>MKRNYILGLDIGITSVGYGIIDYETRDVIDAGVRLFKEANVENNEGRRSKRGARRLKRRRRHRIQRVKKLLFDYNLLTDHSELSGINPYEARVKGLSQKLSEEEFSAALLHLAKRRGVHNVNEVEEDTGNELSTKEQISRNSKALEEKYVAELQLERLKKDGEVRGSINRFKTSDYVKEAKQLLKVQKAYHQLDQSFIDTYIDLLETRRTYYEGPGEGSPFGWKDIKEWYEMLMGHCTYFPEELRSVKYAYNADLYNALNDLNNLVITRDENEKLEYYEKFQIIENVFKQKKKPTLKQIAKEILVNEEDIKGYRVTSTGKPEFTNLKVYHDIKDITARKEIIENAELLDQIAKILTIYQSSEDIQEELTNLNSELTQEEIEQISNLKGYTGTHNLSLKAINLILDELWHTNDNQIAIFNRLKLVPKKVDLSQQKEIPTTLVDDFILSPVVKRSFIQSIKVINAIIKKYGLPNDIIIELAREKNSKDAQKMINEMQKRNRQTNERIEEIIRTTGKENAKYLIEKIKLHDMQEGKCLYSLEAIPLEDLLNNPFNYEVDHIIPRSVSFDNSFNNKVLVKQEENSKKGNRTPFQYLSSSDSKISYETFKKHILNLAKGKGRISKTKKEYLLEERDINRFSVQKDFINRNLVDTRYATRGLMNLLRSYFRVNNLDVKVKSINGGFTSFLRRKWKFKKERNKGYKHHAEDALIIANADFIFKEWKKLDKAKKVMENQMFEEKQAESMPEIETEQEYKEIFITPHQIKHIKDFKDYKYSHRVDKKPNRELINDTLYSTRKDDKGNTLIVNNLNGLYDKDNDKLKKLINKSPEKLLMYHHDPQTYQKLKLIMEQYGDEKNPLYKYYEETGNYLTKYSKKDNGPVIKKIKYYGNKLNAHLDITDDYPNSRNKVVKLSLKPYRFDVYLDNGVYKFVTVKNLDVIKKENYYEVNSKCYEEAKKLKKISNQAEFIASFYNNDLIKINGELYRVIGVNNDLLNRIEVNMIDITYREYLENMNDKRPPRIIKTIASKTQSIKKYSTDILGNLYEVKSKKHPQIIKKG[2x];>SMRKTIERLLNSELSSNSIAVRTGVSQAVISKLRNGKKELGNLTLNSAEKLFEYQKEMEKVDTWIVYRGRTADMNKSYIAEGSTYEEVYNNFVDKYGYDVLDEDIYEIQLLKKNGENLDDYDVDSDGINNYDKLDEFRESDYVDLEDYDYRELFENSSSQVYYHEFEITHE[2x]

AcrIIA15 is an anti-CRISPR (Acr) protein that inhibits Staphylococcus aureus Cas9 (SaCas9). The AcrIIA15 protein, consisting of 170 amino acids, is comprised of two domains: an N-terminal domain (NTD) from residues 1 to 56, which contains a HTH motif resembling a transcriptional repressor, and a C-terminal domain (CTD) from residues 57 to 170. AcrIIA15, by combining the HTH domain and Cas9 inhibitory domain within a single protein, exhibits dual functionality as a bi-functional anti-CRISPR protein capable of both transcriptional repression and CRISPR-based cleavage inhibition. Our structural and biochemical studies demonstrate that AcrIIA15 functions as a dimer to simultaneously inhibit both anti-CRISPR operon transcription and SaCas9-sgRNA DNA recognition.

To address this, we reconstituted the SaCas9-sgRNA-AcrIIA15-IR quaternary complex by incubating these four components together, followed by SEC. We then determined its cryo-EM structure at a resolution of 3.82 Å. Although the resolution of this structure is not high, it is sufficient to reveal the relative locations of all subunits. In this quaternary complex, one AcrIIA15 dimer binds one IR DNA via its HTH domains, while the two CTD domains of the dimer bind two different SaCas9-sgRNA complexes. The interactions between IR1 and AcrIIA15NTD, and between SaCas9-sgRNA and AcrIIA15CTD in this complex are the same as the ones that we observed in their individual structures. However, a structural comparison of this quaternary complex with the AcrIIA15-DNA complex revealed that the position of the AcrIIA15 CTD relative to its NTD is shifted from its location in the dimer:IR1 structure. Although the DNA and HTH domains were well-aligned, both CTD domains are rotated away to accommodate SaCas9 in the quaternary complex. This indicates that the AcrIIA15 dimer undergoes a significant conformational change upon binding to Cas9. Additionally, the short loop connecting the NTD and CTD of AcrIIA15 is flexible, enabling the structural rearrangement of AcrIIA15 in distinct states. Due to the presence of two inverted repeats located upstream of the promoter region, we posit that two AcrIIA15 dimers together with four SaCas9-sgRNA effectors could simultaneously bind to the AcrIIA15 promoter region.> MVDINLFREEKGNNPEIIRESQRRRFASVEIVDEIIKLDKEWRQRQFEVDSFRKEFNKLNKQVAQLKIKKEDASEIIQQTEKNKQDSTAKEAEVREAYAALKAKLEQVG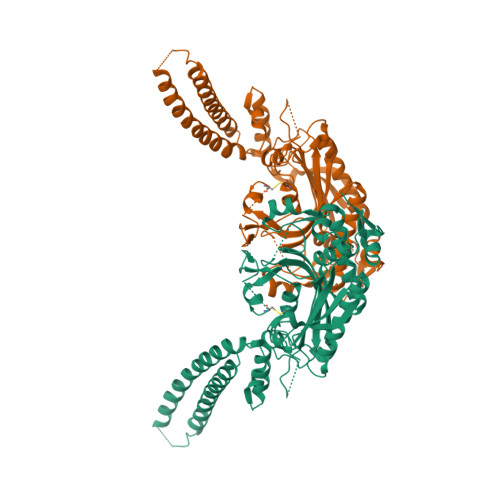NLVHDSVPVDKDEANNLVIKLWGEKRFSTPGLKLKNHVDLVELLGIADTKRGAEIAGARGFFLKGDGLMLNQALINFGLTFLKKRGFTGLQPPFFMRKDVMAKCAQLAQFDEELYKVTGEGDDKYLIATAEQPLCAYHIDEWIHPTELPLRYAGYSSCFRKEAGSHGRDTLGIFRVHQFEKIEQFCITGPNENASWEMLDEMMKNSEDFYQALKLPYQIVSIVSGALNDAAAKKYDLEAWFPSSETFRELVSCSNCTDYQARRLEIRYGQKKSNEQTKQYVHMLNSTLTATERTICCILENYQREDGVDIPEVLQPFMGGETFLPFKAKPVVADTKGKKSKAAAALE> AERPTLPIPDLLTTDARNRIQLTIGAGQSTFGGKTATTWGYNGNLLGPAVKLQRGKAVTVDIYNQLTEETTLHWHGLEVPGEVDGGPQGIIPPGGKRSVTLNVDQPAATCWFHPHQHGKTGRQVAMGLAGLVVIEDDEILKLMLPKQWGIDDVPVIVQDKKFSADGQIDYQLDVMTAAVGWFGDTLLTNGAIYPQHAAPRGWLRLRLLNGCNARSLNFATSDNRPLYVIASDGGLLPEPVKV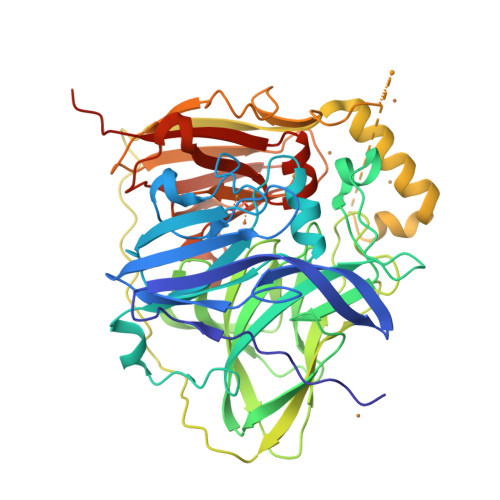SELPVLMGERFEVLVEVNDNKPFDLVTLPVSQMGMAIAPFDKPHPVMRIQPIAISASGALPDTLSSLPALPSLEGLTVRKLQLSMDPMLDMMGMQMLMEKYGDQAMAGMDHSQMMGHMGHGNMNHMNHGGKFDFHHANKINGQAFDMNKPMFAAAKGQYERWVISGVGDMMLHPFHIHGTQFRILSENGKPPAAHRAGWKDTVKVEGNVSEVLVKFNHDAPKEHAYMAHCHLLEHDDTGMMLGFTVLQGDHGLSAWSHPNFEK> SMALGPFPAMENQVLVIRIKIPNSGAVDWTVHSGPQLLFRDVLDVIGQVLPEATTTAFEYEDEDGDRITVRSDEEMKAMLSYYYSTVMEQQVNGQLIEPLQIFPRA;> SMGHSNRQSDVRIKFEHNGERRIIAFS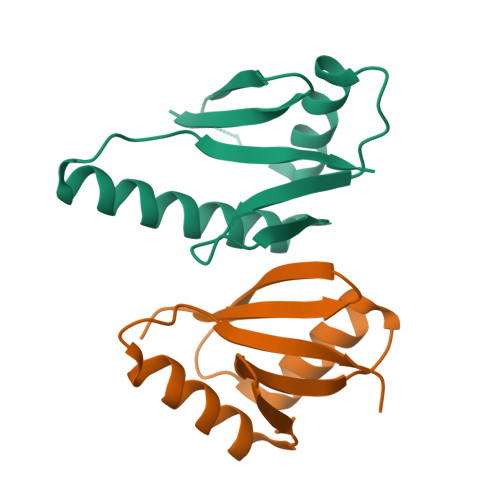RPVKYEDVEHKVTTVFGQPLDLHYMNNELSILLKNQDDLDKAIDILDRSSSMKSLRILLLSQD> AGLNKDQKRRAEQLTSIFANGTTEIQYGYVERLDDGRGYT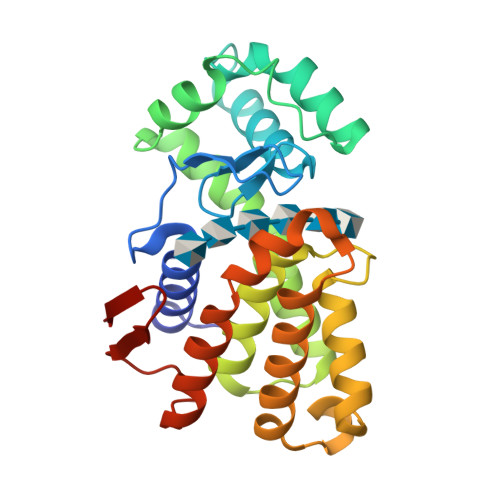CGRAGFTTATGDALEVVEVYTKAVPNNKLKKYLPELRRLAKEESDDTSNLKGFASAWKSLANDKEFRAAQDKVNDHLYYQPAMKRSDNAGLKTALARAVMYDTVIQHGDGDDPDSFYALIKRTNKKAGGSPKDGIDEKKWLNKFLDVRYDDLMNPANHDTRDEWRESVARVDVLRSIAKENNYNLNGPIHVRSNEYGNFVIK> MHHHHHHENLYFQGTKDLNTLVSELPEIYQTIFGHPEWDGDAARDCNQRLDLITEQYDNLSRALGRPLNVLDLGCAQGFFSLSLASKGATIVGIDFQQENINVCRALAEENPDFAAEFRVGRIEEVIAALEEGEFDLAIGLSVFHHIVHLHGIDEVKRLLSRLADVTQAVILELAVKEEPFYWGVSQPDDPRELIEQCAFYRLIGEFDTHLSPVPRPMYLVSNHRVLINDFNQPFQHWQNQPYAGAGLAHKRSRRYFFGEDYVCKFFYYDMPHGILTAEESQRNKYELHNEIKFLTQPPAGFDAPAVLAHGENAQSGWLVMEKLPGRLLSDMLAAGEEIDREKILGSLLRSLAALEKQGFWHDDVRPWNVMVDARQHARLIDFGSIVTTPQDCSWPTNLVQSFFVFVNELFAENKSWNGFWRSAPVHPFNLPQPWSNWLYAVWQEPVERWNFVLLLALFEKKAKLPSAEQQRGATEQWIIAQETVLLELQSRVRNESAGSEALRGQIHTLEQQMAQLQSAQDAFVEKAQQPVEVSHELTWLGENMEQLAALLQTAQAHAQADVQPELPP

The chain length of the O9a O-PS is tightly regulated by the WbdD enzyme. WbdD first phosphorylates the terminal non-reducing mannose of the O-PS and then methylates the phosphate, stopping polymerization. The 82 kDa WbdD protein from E. coli O9a comprises 708 residues and contains three domains, an N-terminal methyltransferase (MTase) domain, a kinase domain and a C-terminal domain (residues 460–708) that includes predicted coiled-coil motifs. WbdD is an unusual enzyme since it combines both a phosphate-methyltransferase and a sugar kinase activity.

Here, we report the 2.2 Å crystal structure of the bi-functional catalytic domain of the WbdD protein from E. coli O9a. The full-length WbdD protein was not tractable for biophysical characterization but a 63 kDa fragment, comprising residues 1–556 (WbdD556), could be expressed, purified and crystallized. The WbdD556 structure has an elongated shape with an N-terminal MTase domain (residues 1–210) directly adjacent to the kinase domain (residues 211–459). WbdD556 is a trimer in the crystal, consistent with its status in solution as judged by gel-filtration. The C-terminal α-helix (αV) (residues 459–473) of each monomer wraps around the crystallographic threefold axis forming a trimeric bundle reminiscent of a coiled-coil. Residues 474–556 are disordered, possibly because of packing constraints but are predicted to be helical. The S-adenosylmethionine (SAM) binding site located on top of the β-sheet. Positively-charged residues (R203, H132 and H133) cluster around the electrophilic methyl group, consistent with a phosphate binding site (arising from the phosphorylated sugar substrate). The pocket is occupied by sulphate in the WbdD556 structure, these crystals were grown from ammonium sulphate solutions whereas the pocket is empty (with the loops disordered) in WbdD459 crystals which were grown from a non-sulphate-containing solution. Our data show the two domains are arranged to produce the unique methyl-phosphate modification on the 3-OH of the non-reducing terminal mannose.> GAFLDKPKMEKHNAQGQGNGLRYGLSSMQGWRVEMEDAHTAVIGLPS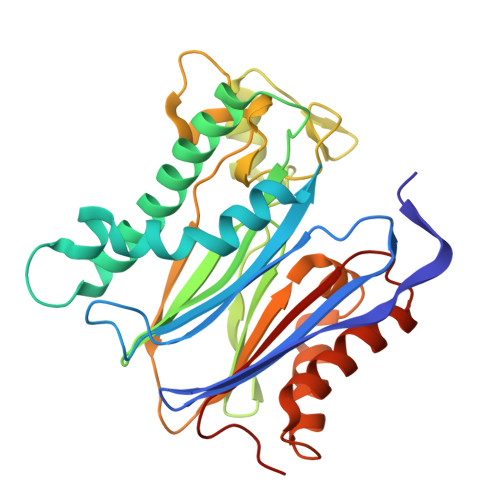GLESWSFFAVYDGHAGSQVAKYCCEHLLDHITNNQDFKGSAGAPSVENVKNGIRTGFLEIDEHMRVMSEKKHGADRSGSTAVGVLISPQHTYFINCGESRGLLCRNRKVHFFTQDHKPSNPLEKERIQNAGGSVMIQRVNGSLAVSRALGDFDYKCVHGKGPTEQLVSPEPEVHDIERSEEDDQFIILACDGIWDVMGNEELCDFVRSRLEVTDDLEKVCNEVVDTCLYKGSRDNMSVILICFPNAPKV>MKRVLVTLGAVAALATGAVAGGGAHWGYSGSIGPEHWGDLSPEYLMCKIGKNQSPIDINSADAVKACLAPVSVYYVSDAKYVVNNGHTIKVVMGGRGYVVVDGKRFYLKQFHFHAPSEHTVNGKHYPFEAHFVHLDKNGNITVLGVFFKVGKENPELEKVWRVMPEEPGQ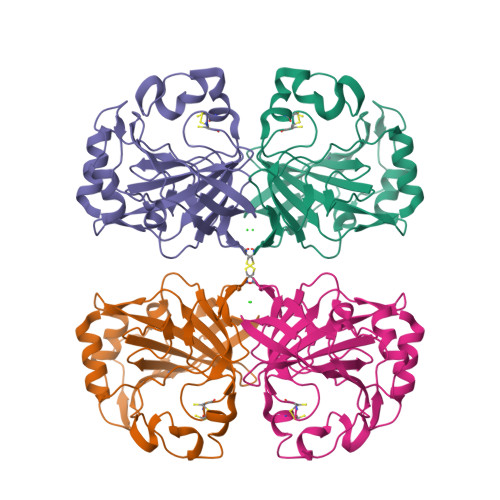KRHLTARIDPEKLLPENRDYYRYSGSLTTPPCSEGVRWIVFKEPVEMSREQLEKFRKVMGFDNNRPVQPLNARKVMK[2x]> ADIGSNIFYAGDATKSNYFRIPSLLALDSGTVIAAADARYGGTHDAKSKINTAFAKSTDGGKTWGQPTLPLKFDDYVAKNIDWPRDSVGKNVQIQGSASYIDPVLLEDKETHRVFLFADMMPAGIGSSNASVGSGFKEVDGKKYLKLHWKDDAAGTYDYSVRENGTIYNDTTNSATEYSVDGEYNLYKNGNAMLCKQYDYNFEGTKLLETQTDTDVNMNVF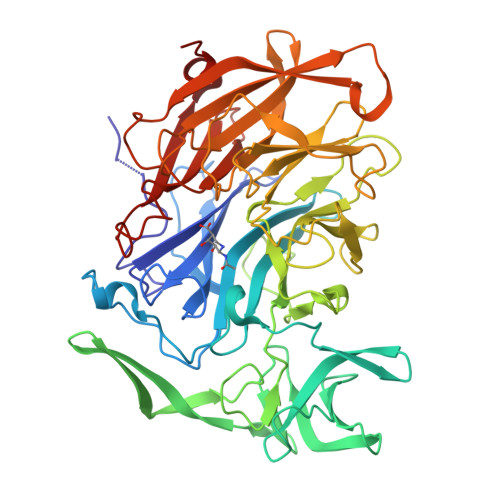YKDADFKVFPTTYLAMKYSDDEGETWSDLQIVSTFKPEESKFLVLGPGVGKQIANGEHAGRLIVPLYSKSSAELGFMYSDDHGNNWTYVEADQNTGGATAEAQIVEMPDGSLKTYLRTGSGYIAQVMSTDGGETWSERVPLTEIATTGYGTQLSVINYSQPVDGKPAILLSAPNATNGRKNGKIWIGLISETGNSGKDKYSVDWKYCYSVDTPQMGYSYSCLTELPDGEIGLLYEKYDSWSRNELHLKNILKYERFNIDELKVQP In this study, we used the enzyme involved in the penultimate step of riboflavin biosynthesis as a test specimen to benchmark a recently installed microscope and determine if other protein complexes could reach a resolution of 1.5 Å or better, which so far has only been achieved for the iron carrier ferritin. Of these, AaLS from the hyper-thermophilic bacterium Aquifex aeolicus forms a 1 MDa spherical capsid of 60 identical subunits with icosahedral symmetry.

Using state-of-the-art microscope and detector hardware as well as the latest software techniques to overcome microscope and sample limitations, a 1.42 Å map of Aquifex aeolicus lumazine synthase (AaLS) was obtained from a 48 h microscope session. The final 3D reconstruction of AaLS consisted of 470 878 particles. This 1.43 Å map was slightly improved by Ewald sphere correction to 1.42 Å [Figs. 2(a), and S1(a) and S1(b) of the supporting information]. The half maps from Ewald sphere correction were subsequently used for atomic model refinement using the 1.60 Å crystal structure of AaLS as a starting model. A mask-normalized Fo − Fc-generated difference map was then used to identify peaks within 0.5 Å of hydrogen atoms in a reduced model, followed by manual curation which resulted in 552 hydrogens. Thus, we were able to identify ∼46% of all putative protein hydrogen atoms from the map of AaLS at this resolution [Figs. 2(b) and 2(c)]. About 70% of hydrogen atoms could be located in maps at 1.19 and 1.25 Å resolution compared with only ∼17% at 1.84 Å resolution. Several of the water molecules identified displayed hydrogen densities adjacent to the central oxygen atom [Fig. 2(d)]. Finally, we observed the density for a tetrahedral-shaped ligand. This was built as a phosphate ion and is consistent as a bi-product of lumazine synthesis and in proximity to Arginine 127, a highly conserved residue in this family of proteins [Fig. 2(e)]. At pH 7.5 the phosphate ion is expected to be mostly in the HPO4−2 proton­ation state, though we did not observe positive density for any hydrogens. The structure we obtained from a 48 h session at 1.42 Å is to date the only sub-1.5 Å structure of a complex other than apoferritin.

> MQIYEGKLTAEGLRFGIVASRFNHALVDRLVEGAIDCIVRHGGREEDITLVRVPGSWEIPVAAGELARKEDIDAVIAIGVLIRGATPHFDYIASEVSKGLANLSLELRKPITFGVITADTLEQAIERAGTKHGNKGWEAALSAIEMANLFKSLRWSHPQFEK> 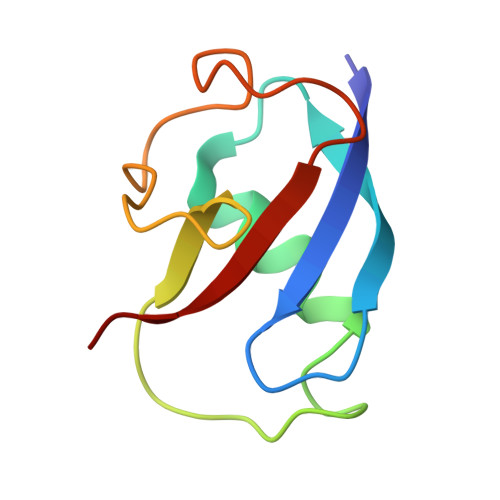SAFPVHAAFEKDFLVQLVVVDLNDSMDQVAEKVAYHCVNRRVAPREGVMRVRKHRSTELFPRDMTIAESGLNPTEVIDVVFEE> GAMDDSSLQKVELQTDVYMVCLQHALSTENFEVMGLLIGNFACGIAKISAVIILRRLDKKKDRVEISSEQLLKAAAEAERLTVELNRPMRVLGWYQSQPHITVCPSHVDVRTQATYQTMDHSFVGLIFSVFSEGKESKEHEIFLNCFQSDNGEATEIPLEIVHTPDISDRCLRTMTDLSKILVQEEEDMAEACKDHPDVLASIHNNAVRTRALIHITDIITKPLVQTFEKRIA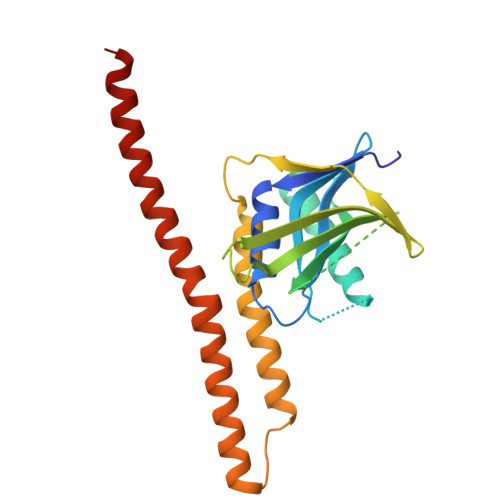LNKLRATHLQRQLQELQKMCNG>GMEEDIACVKDLVSKYLADNERLSRQKLAFLVQTEPRMLLMEGLKLLSLCIEIDSCNANGCEHNSEDKSVERILHDHGILTPSLCFVVPDGYKLTGNVLILLECFVRSSPANFEQKYIEDFKKLEQLKEDLKTVNISLIPLIDGRTSFYNEQIPDWV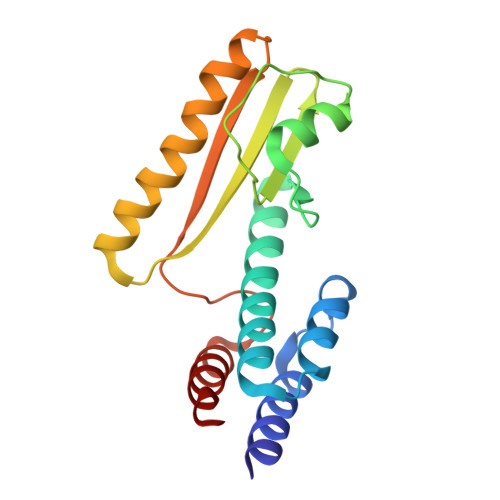NDKLRDTLFSLLRY[2x]>[4x]MREKDYVVIIGSANIDVAGYSHESLNYADSNPGKIKFTPGGVGRNIAQNLALLGNKAWLLSAVGSDFYGQSL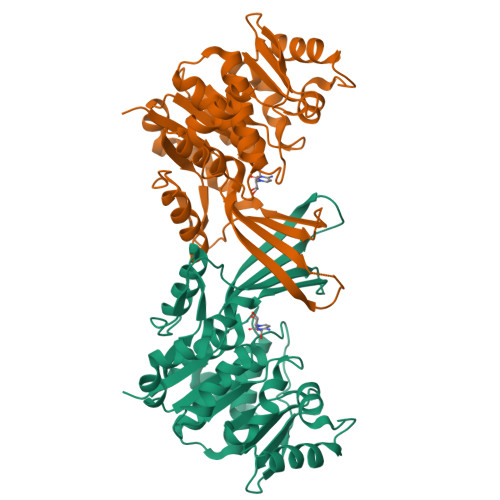LTQTNQSGVYVDKCLIVPGENTSSYLSLLDNTGEMLVAINDMNISNAITAEYLAQHREFIQRAKVIVADCNISEEALAWILDNAANVPVFVDPVSAWKCVKVRDRLNQIHTLKPNRLEAETLSGIALSGRDDVAKVAAWFHQHGLNRLVLSMGGDGVYYSDIRGENGWSAPIKTNVINVTGAGDAMMAGLASCWVDGMPFAESVRFAQGCSSMALSCEYTNNPDLSIANVISLVENAECLN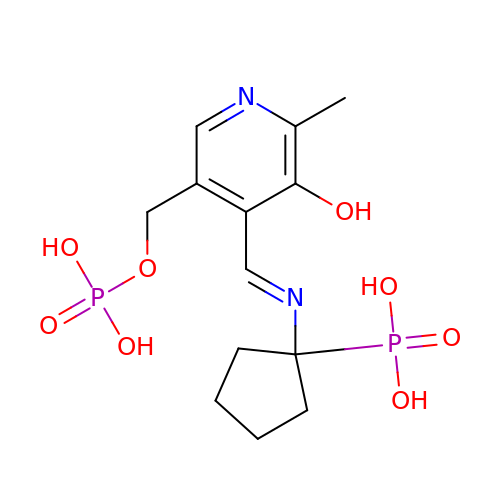1-[((1E)-{3-HYDROXY-2-METHYL-5-[(PHOSPHONOOXY)METHYL]PYRIDIN-4-YL}METHYLENE)AMINO]CYCLOPENTYLPHOSPHONIC ACID | C13 H20 N2 O8 P2 | NPYNJFSRGFRPCR-VIZOYTHASA-N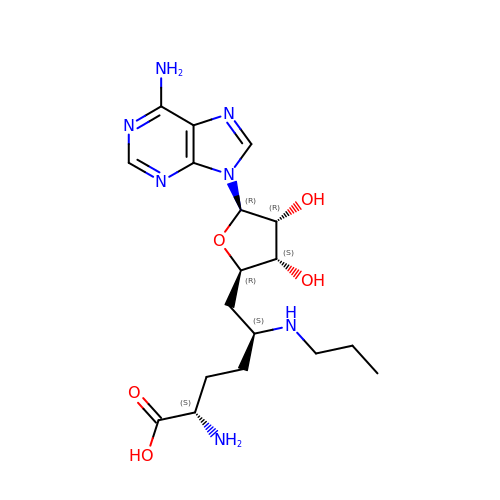(2S,5S)-2-amino-6-[(2R,3S,4R,5R)-5-(6-amino-9H-purin-9-yl)-3,4-dihydroxytetrahydrofuran-2-yl]-5-(propylamino)hexanoic acid | C18 H29 N7 O5 | ZDIZXAAADLAUDS-GTAFEMJLSA-N[2-(5-amino-4-cyano-1H-pyrazol-1-yl)-5-(trifluoromethyl)phenyl](hydroxy)oxoammonium 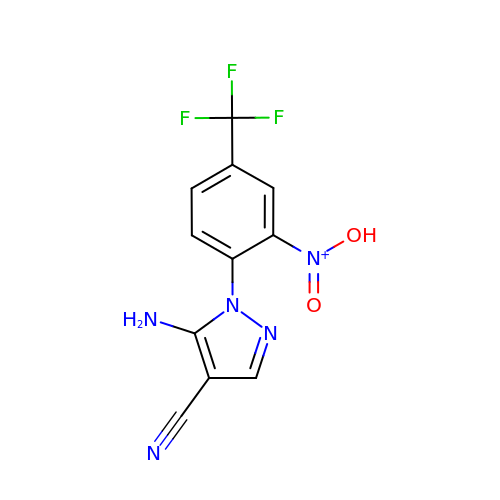| C11 H7 F3 N5 O2 | XSUKDZBLRKXERL-UHFFFAOYSA-N> MAHHGVSGLVGKLVTQLEVNCDADIFYKIVKHHEEVPNVIPHFFTGV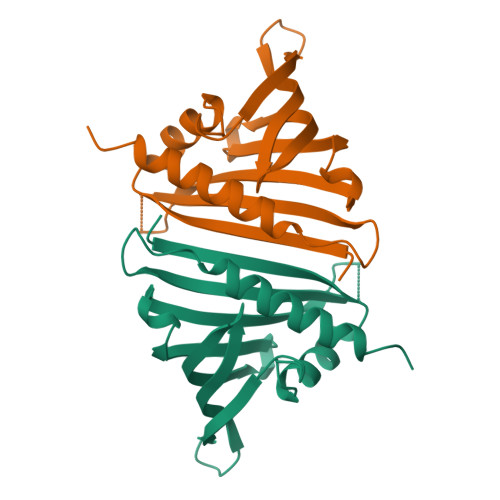QVTKGDGLVSGSIKEWNYVLEGKAMTAVEETTHADETRTLTHHITEGDAMKDYKKFDVIVETNPKPNGHGSVVTYSIVYEKINEDSPAPFDYLKFFHQNIVDMSAHICSSA> AAGCAGACCTGACTGCACTCA;> AGTCA;> TCTGAGTGC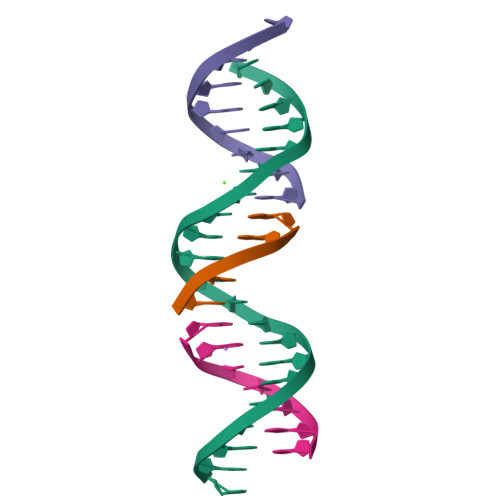;> GGTCTGC>[2x]MASSHHHHHHLEVLFQGPSALRSTKGLVALVTGGASGLGRGAAENLLKHGAKVAILDLPSSAGAEVAKELGGDCIFTPASVTAASEVKSALADVKKKFGRLDVAVNCAGIAYSFKLFNVKKKKLCDLESVRKTLDVNVMGYFTVAAHAAELFAENEKDEMGQRGVIINTASIAAFDGQAGQSAYSASKGAIVGMTLPLARDFADDGIRVVTIAPGIFDTPMMASFPDKVRNF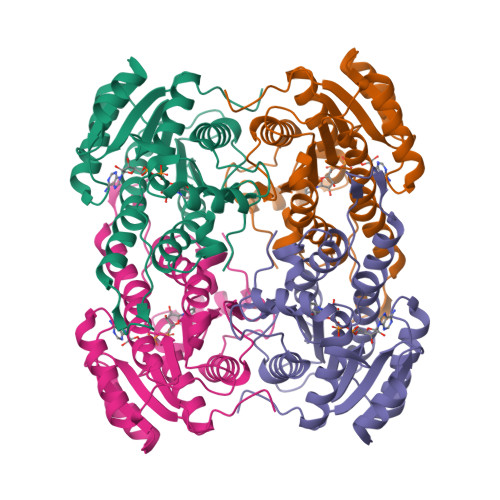LIGLVPNPKRFGVPEEYGALVRHIIENRYLNGEVIRLDGALRMPA> ASMTGGQQMGRGSGSEFMENETHYAEAVIDNGAFGTRTIRFETGRLARQAAGSAVAYLDDDTMVLSATTASKNPKDQLDFFPLTVDVEERMYAAGKIPGSFFRREGRPSEDAILTCRLIDRPLRPSFKKGLRNEIQVVATIMALNPDHLYDVVAINAASASTQLAGLPFSGPIGGVRVALIRGQWVAFPTHTELEDAVFDMVVAGRVLEDGDVAIMMVEAEATEKTIQLVKDGAEAPTEEVVAAGLDAAKPFIKVLCKAQADLAAKAAKPTGEFPVFLDYQDDVLEALSAAVRPELSAA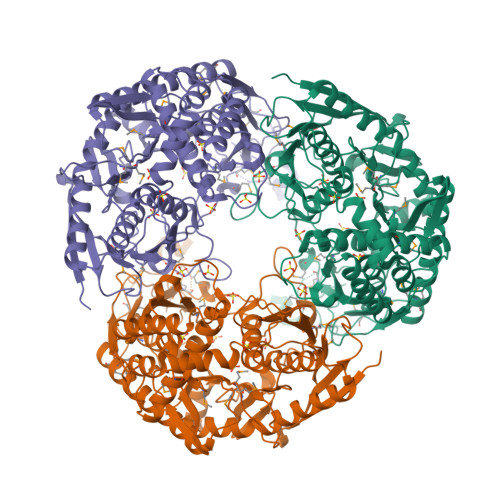LTIAGKQDREAELDRVKALAAEKLLPEFEGREKEISAAYRALTKSLVRERVIAEKKRIDGRGVTDIRTLAAEVEAIPRVHGSALFERGETQILGVTTLNMLRMEQQLDTLSPVTRKRYMHNYNFPPYSVGETGRVGSPKRREIGHGALAERAIVPVLPTREEFPYAIRQVSEALGSNGSTSMGSVCASTMSLLNAGVPLKAPVAGIAMGLISQEINGETHYVALTDILGAEDAFGDMDFKVAGTKEFVTALQLDTKLDGIPASVLAAALKQARDARLHILDVMMEAIDTPDEMSPNAPRIITVKIPVDKIGEVIGPKRQMINQIQEDTGAEITIEDDGTIYIGAADGPAAEAARATINGIANPTSPEVGERILGSVVKTTTFGAFVSLLPGKDGLLHISQIRKLAGGKRVENVEDVLGVGQKVQVEIAEIDSRGKLSLIPVIEGEEAASDEKKDDAEQ> MKHMPRKMYSCAFETTTKVEDCRVWAYGYMNIEDHSEYKIGNSLDEFMAWVLKVQADLYFHNLKFAGAFIINWLERNGFKWSADGLPNTYNTIISRMGQWYMIDICLGYKGKRKIHTVIYDSLKKLPFPVKKIAKDFKLTVLKGDIDYHKERPVGYKITPEEYAYIKNDIQIIAEALLIQFKQGLDRMTAGSDSLKGFKDIITTKKFKKVFPTLSLGLDKEVRYAYRGGFTWLNDRFKEKEIGEGMVFDVNSLYPAQMYSRLLPYGEPIVFEGKYVWDEDYPLHIQHIRCEFELKEGYIPTIQIKRSRFYKGNEYLKSSGGEIADLWLSNVDLELMKEHYDLYNVEYI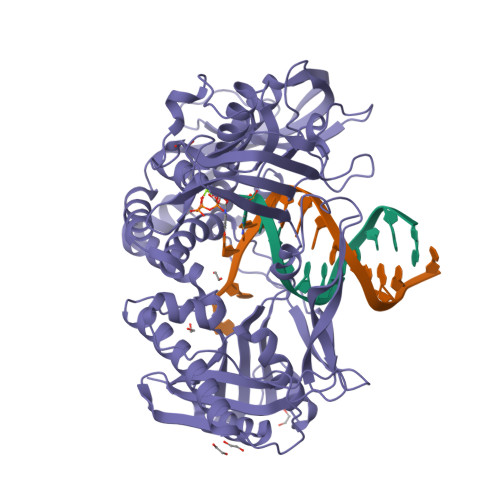SGLKFKATTGLFKDFIDKWTYIKTTSEGAIKQLAKLMLNSLYGKFASNPDVTGKVPYLKENGALGFRLGEEETKDPVYTPMGVFITAWARYTTITAAQACYDRIIYCDTDSIHLTGTEIPDVIKDIVDPKKLGYWAHESTFKRAKYLRQKTYIQDIYMKEVDGKLVEGSPDDYTDIKFSVKCAGMTDKIKKEVTFENFKVGFSRKMKPKPVQVPGGVVLVDDTFTIK>[2x]MTAKDIATEESKIRAYAQWMEITIFVVNSNFKVEGAYLRWGKFHVPGDKDKEISPSQINGTIIKDEDSYTIASCGRENASSGTEGGFSLYDGDKLVFEYYWDCPWSGSNSDELTVKDKENYTVIKKGGGSPSGAMGNIFITVVKKSLEHHHHHH

Here we report the discovery of a two-component WCR-active protein, AfIP-1A/1B, from the Gram-negative bacterium Alcaligenes faecalis. While the amino acid sequences of these proteins bear little similarity to known corn rootworm-active proteins, cross-resistance evaluations, competitive binding studies and comparison of protein structures indicate that AfIP-1A/1B kills WCR through a mechanism that is similar to Cry34Ab1/Cry35Ab1. AfIP-1A represents a 441 nucleotide gene that encodes the AfIP-1A protein of 146 amino acids with a deduced molecular mass of about 16.1 kDa and predicted pI of 4.8. Cell lysates of cultures of all transformations were inactive against WCR in diet assays when each protein was assayed alone but proved insecticidal when both proteins were present.

We were able to determine structure of AfIP-1A(I20M, T135M), an insecticidal variant of AfIP-1A, to 1.8 Å resolution by x-ray crystallography. In the P21 crystal form the structure of AfIP-1A is a dimer with monomers consisting of 11 beta strands with one short α-helix at the N-terminus. The N-terminal 8 residues in both monomers are missing from the model due to the lack of electron density in this region, indicative of a highly flexible N-terminal polypeptide. Three surface loops, residues 77–82, 103–109 and 128–131 are also highly mobile with weak or missing electron density. The monomer structures are virtually identical except for the above 3 surface loops and the flexible N-terminal polypeptide segment. Superposition of the two monomers on Cα atoms gave an RMSD of 0.0906 Å (calculated with LSQKAB28) over 118 residues. The superimposed structures reveal a high degree of structural similarity between Cry34Ab1 and AfIP-1A. The RMS deviation between main chain atoms of the β-sandwich (105 residues) is 1.92 Å. The major structural divergence is observed within the region spanning AfIP-1A Pro46-Ile62 and Cry34Ab1 Thr33-Asn37. Cry34Ab1 has a simple four amino acid coiled region connecting β3 and β4 whereas AfIP-1A contains a three residue turn, five residue β strand, and five residue α helix in the structurally equivalent region.> MDIKYKLASYRICSPEETFEKIQEALKKIETVEIKNIQHLDKVNIPVYYLKRRVVVDGKEGIAIHYGKGANDIQAKVSACMEAIERFSASYDKNKVKEKPDNPINVEDLI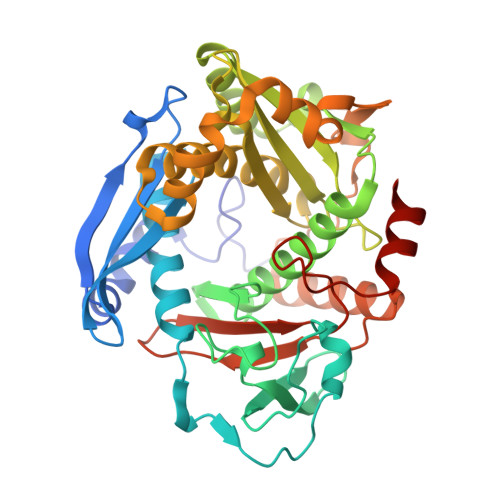LPQYADKNVKEWVEGIDIINNETIDVPADAVFYPTSGKLFRGNTNGLASGNNLDEAILHATLEIIERDAWSLADLARKIPTKINPEDAKNPLIHELIEKYEKAGVKIILKDLTSEFEIPVVAAISDDLSKNPLMLCVGVGCHLHPEIAILRALTEVAQSRASQLHGFRRDAKLREEFTSKIPYERLKRIHRKWFEFEGEINIADMPNNARYDLKKDLKFIKDKLSEFGFDKLIYVDLNKVGVDAVRVIIPKMEVYTIDRDRLSRRAFERVKKLYY> SNAELNSIGVTVGDLANPFFVQITKGVELEARKLAGDKVKVTLVSSGYDLGQQVAQIDNFIAAKVDMIILNAADSKGIGPAVKRAKDAGIVVVAVDVAAEGADATITSDNTQAGAMACKYISDRLKEKGNVVIINGPPVSAIQNRVEGCESEFKKYPDIKVLSSNQNAKGSREGGLEVMTSLLAVNPKIDGVFAINDPTAIGADLAAKQAQRNEFFIVGVDGSPDAEEALKRGGNTLFVATPAQDPQVMASKAVEVGYGILQGNPAPKDPILIPVTLIDKN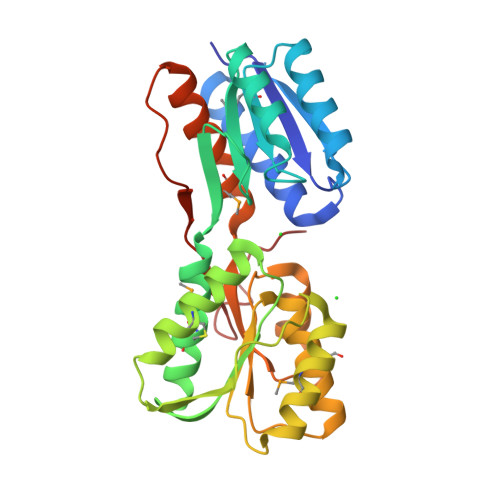NISTYKGWTMK>GCGCCGGUUAGGCAGUGGUGGGUGGUGUGGAGGAGUAGCUGUCCGGCGC[2x]

Beetroot is a homodimeric in vitro selected RNA that binds and activates DFAME, a conditional fluorophore derived from GFP. It is 70% sequence-identical to the previously characterized homodimeric aptamer Corn, which binds one molecule of its cognate fluorophore DFHO at its interprotomer interface. Each protomer comprises two duplex segments (P1 and P2) separated by an irregular junction (J1/2) and a mixed connectivity quadruplex. The latter has three canonical G-quartet tiers (T1, T2, and T3) and one mixed-composition (G•U•A•A) tier (T4).

Remarkably, the double mutation that converts this Watson-Crick pair into the wobble base pair U16•G38 (A16U, U38G) results in three times higher activation of DFHO, compared to the wild-type Beetroot. Moreover, this mutant (hereafter, Wobble Beetroot) activates DFAME fluorescence only 25% as much as the wild-type. Thus, replacement of a single P2 base pair from A•U to U•G resulted in a ~ 12-fold switch of fluorescence activation from DFAME to DFHO. To elucidate the structural basis of the selectivity switch from DFAME to DFHO of Wobble Beetroot, we next determined its co-crystal structure bound to DFHO at 2.85 Å resolution. The overall structure of Wobble Beetroot bound to DFHO is similar to those of the wild-type Beetroot fluorophore complexes (r.m.s.d. of 2.10 Å for C1’ pairs between the Wobble Beetroot-DFHO and the wild-type Beetroot-DFHO complexes without J1/2). However, the DFHO bound to Wobble Beetroot has rotated ~ 30° on its plane when compared to its pose when bound to wild-type Beetroot. In addition, the conformation of the carbaldehyde oxime substituent is also reversed. Thus, this substituent stacks completely on the nucleobase of A34 in Wobble Beetroot, while it does not stack directly on any of the nucleobases of T4 in the wild-type. Comparable to the other complexes of Beetroot–ligand here reported, the wobble Beetroot–DFHO binding only buries 37% of the solvent-accessible surface area of the ligand. Our newly engineered variant, Wobble Beetroot, has a dimerization interface unchanged from that of its parental aptamer.>[2x]SGQGALDRVALGGLLNTLAARVHCTSGPCGKCLSVDDLLALGRPEEPGHLARLSAAAALYLSDPEGTCEDIRAGRWASRADHLLALL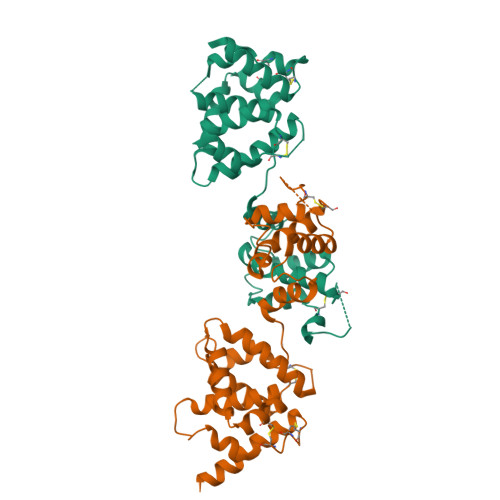EGPKALAPGLSRLLQRIQAQTTGQPSAGEACVDPPQLLREAGVAGAPGSPGPVLATLLEHVGRGSCFHTLPTPQYFVDFVFQQSHGNTPNISVAELAALMQRLGVGGVTETHSDHHHQEKRVNRQGPTPLTAPNSSSDTWDTVCLSARDVMAVYGLSEQTGVTPEAWAQLSPALLQQQLSGACSPQPSHPAQNQLSQAEK> A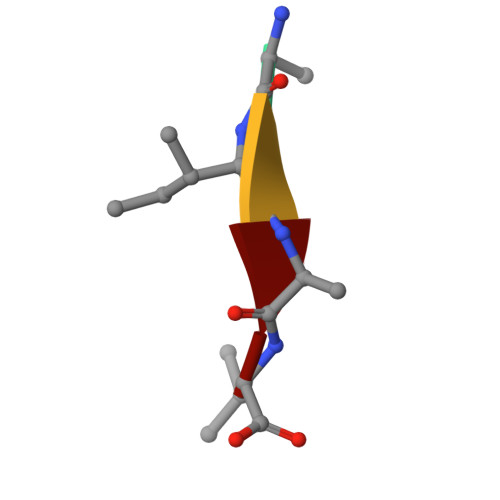IAV>[2x]MYEALLVVFLIVAIGLVGLIMLQQGKGADMGASFGAGASATLFGSSGSGNFMTRMTALLATLFFIISLVLGNINSNK;>[2x]MAKQPGLDFQSAKGGLGELKRRLLFVIGALIVFRIGSFISIFALGIMPYISASIIIQLLTVVHPTLAEIKKEGESGRRKISQYTRYGTLVLAIFQSIGIATGLPNMPGMQGLVINPGFAFYFTAVVSLVTGTMFLMWLGE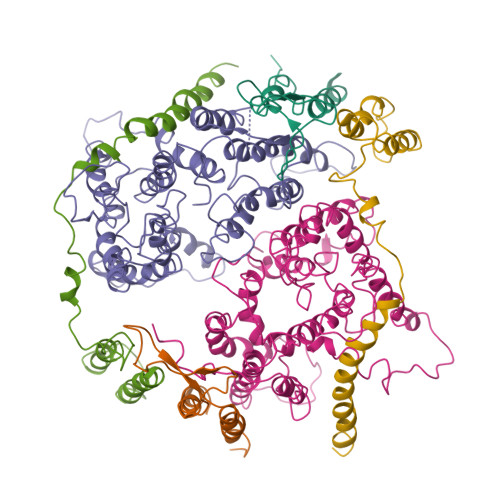QITERGIGNGISIIIFAGIVAGLPPAIAHTIEQARQGDLHFLVLLLVAVLVFAVTFFVVFVERGQRRIVVNYAKRQQGRRVYAAQSTHLPLKVNMAGVIPAIFASSIILFPATIASWFGGGTGWNWLTTISLYLQPGQPLYVLLYASAIIFFCFFYTALVFNPRETADNLKKSGAFVPGIRPGEQTAKYIDKVMTRLTLVGALYITFICLIPEFMRDAMKVPFYFGGTSLLIVVVVIMDFMAQVQTLMMSSQYESALKKA;>[2x]MKWVVVVALLLVAIVGNYLYRDIMLPLRALAVVILIAAAGGVALLTTKGKATVAFAREARTEVRKVIWPTRQETLHTTLIVAAVTAVMSLILWGLDGILVRLVSFITGLRF> GSLLSDE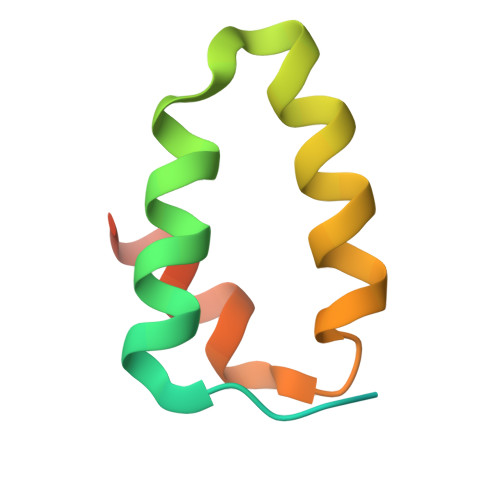HLALLAKYYATVEFTGEQKDALIEKYWEANEAERKAIARAYASLFANDADFIQRLLAHYDMHVS>[2x]GAMGTAGSDLDDFRGLLA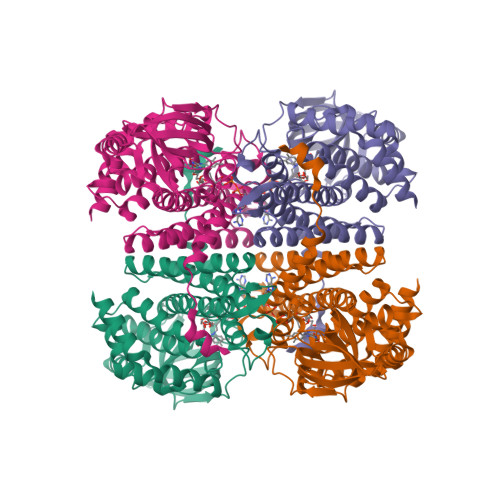KAFDERVVAWTAEAEAQERFPRQLIEHLGVCGVFDAKWATDARPDVGKLVELAFALGQLASAGIGVGVSLHDSAIAILRRFGKSDYLRDICDQAIRGAAVLCIGASEESGGSDLQIVETEIRSRDGGFEVRGVKKFVSLSPIADHIMVVARSVDHDPTSRHGNVAVVAVPAAQVSVQTPYRKVGAGPLDTAAVCIDTWVPADALVARAGTGLAAISWGLAHERMSIAGQIAASCQRAIGITLARMMSRRQFGQTLFEHQALRLRMADLQARVDLLRYALHGIAEQGRLELRTAAAVKVTAARLGEEVISECMHIFGGAGYLVDETTLGKWWRDMKLARVGGGTDEVLWELVAAGMTPDHDGYAAVVGASKA The precursor PdDfsB is cleaved by subtilisin to yield biologically active Slf, and the chemical gradients of both proteins between two growing colonies could be accurately modelled. However, remarkably, the dfsB gene is widely distributed across Gram-positive and to some extent Gram-negative bacterial kingdoms (PFAM entry DUF1706). PdDfsB adopts a four-helical bundle core structure that belongs to the DinB structural superfamily. The most strongly conserved region of PdDfsB is the C-terminal helix, which is present within the mature Slf sequence.

The third, well-populated clade contains exclusively Gram-positive bacteria such as Listeria and some Streptococcus species. During purification of the two Streptococcus DfsB homologues (Streptococcus agalactiae and Streptococcus pneumoniae), both monomers and stable dimers could be identified. We attempted to crystallise both forms independently and only the dimers yielded diffraction-quality crystals. We solved the crystal structure of a S. agalactiae DfsB dimer (SaDfsB) by molecular replacement using a pruned CdDfsB structure as the search model. Interestingly, the source of dimerisation is via the C-terminal helix, which flips out of one monomer and inserts into the other in a mutual fashion.

>[2x]MRGSHHHHHHGSRTYSDKNELKEEVLKSYKKYIAEFNDIPEKLKDLRIDEVDRTPAENLAYQVGWTTLILKWESDEQSGLEVKTPTETFKWNQLGELYQHFTETYASLTIKELTAQLNDNVDAIGNMIDSMSDEVLFKPHMRNWADSATKNAVWEVYKFIHINTVAPFGTFRTKIRKWKKVALK> GHMGGIPLSCVTRQGDLRLGRHLVPHLFEDHAAATPERRALVYNDRAYSYDQLNRAANRIANRLMQAFPELGTDSLVGVRIARSDRLALTVLAIWKIGAAYIPIDPVLPAQRMHDMLDLAGAKALIVDASVAAAEPAVAGMPRIVFDDLVMDDPLLEDNPEVHLSGNDLSYVLFTSGSTGKPKGAMIEHIGMLNNIANKALDLAMDEDSRVAQNASMSFDVSVWQMFIALTKGGTTFVYDDRVVNDIAGLIQRMHTDSLTILEVVPTYLQALVEYMEEHPDCPRPAALTFMMVNGETVDAALLKRWFALCPASKVINAYGPTEASDDITHHIMSPGDEIVNPVPIGRALANFDIYIVDDELRPVPIGTRGEIVVTGVGVGRGYVGMAGVTAQAFVKSPFPDRY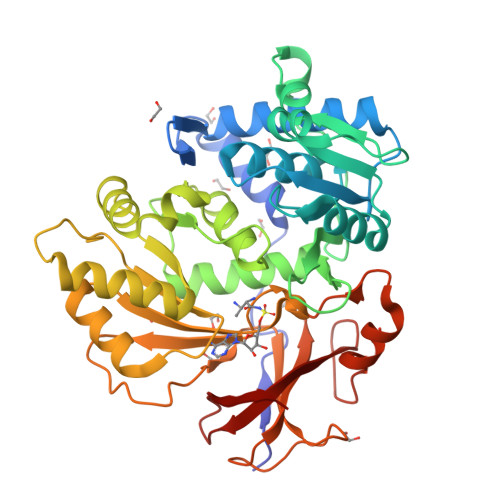KGRLYRTGDLGAMREDGVLMFHGRKD(2E,6E)-12-fluoro-11-(fluoromethyl)-3,7-dimethyldodeca-2,6,10-trien-1-yl trihydrogen diphosphate | C15 H26 F2 O7 P2 | 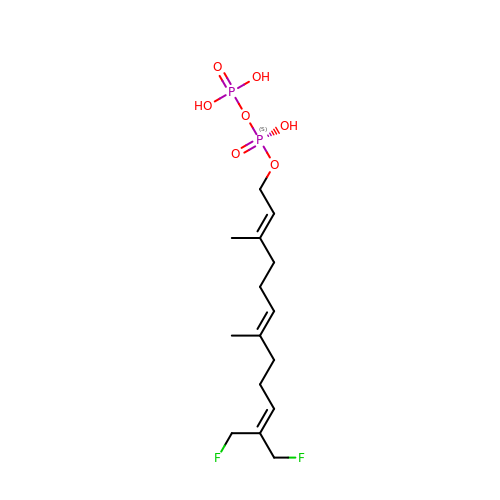PVNRGYDHHSWPHV-HJAIQHMZSA-N>TGAEPQALPSDPLEQALHQAWQAQLGAPPRAGQGFYAAGGDSLRAVHLLATLRQRLSRRVPLQAFAGGPATPEALLELLRQAAPEGDEPEPSAGAAGLSLAERRLWVAQQLAPEDTSYNLLAHLRIVGATADAIEQALRQLLERHVALRRRVETGVDGPQPHALAAHAVPLQRLLASDAVHAERLLEDGVRREGARVFDLAHEAPARLLLVVTRDSARADLLLSVHHYAFDDVSLAVFAAELKTLLDGGRLGVLASTPEQVAARERAALASGRLDRVAERWAERLLPLAKAPGAAPARPEESGGRAGQRLALPVSAAVHAACRALAERTSVSPFSAALQAFAEVLGAELGVDDLLVGVALAGRSRLEMQGLVGCFVNLLPLAVGLRPEQSVEWRLRQVGHDLLELLEHQDVPLECVTQALRQRGASGLPIRIACGAHNGRAAPAVDAGVRVEADFIPVPGARLDLTLWLEDQPQGWLAVWTGVSAIFDLHRIERLHQAWERRLLANAGEPISKRMSPEG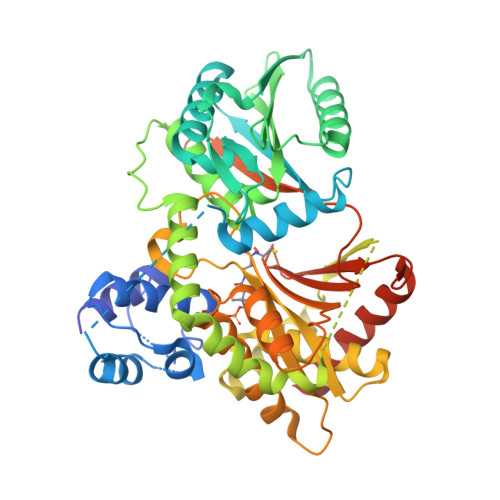CNAS[4x]4-[4-[(4,4-dimethylpiperidin-1-yl)methyl]phenyl]-9-[6-(methylamino)pyrimidin-4-yl]-1,4,9-triazaspiro[5.5]undecan-2-one | C27 H39 N7 O | 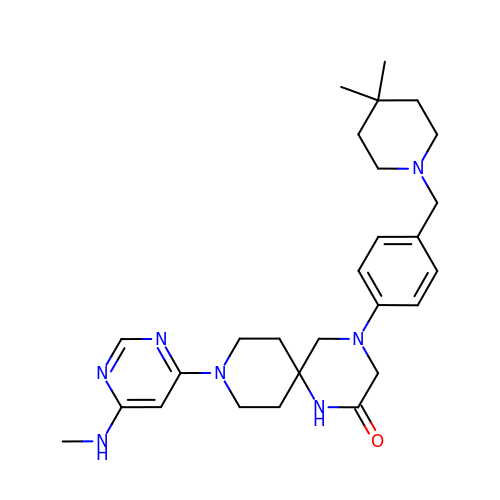JNZJZYBWYKPHFG-UHFFFAOYSA-N4-methyl-6-{[(3R,4R)-4-{[5-(4-methylpyridin-2-yl)pentyl]oxy}pyrrolidin-3-yl]methyl}pyridin-2-amine | C22 H32 N4 O | 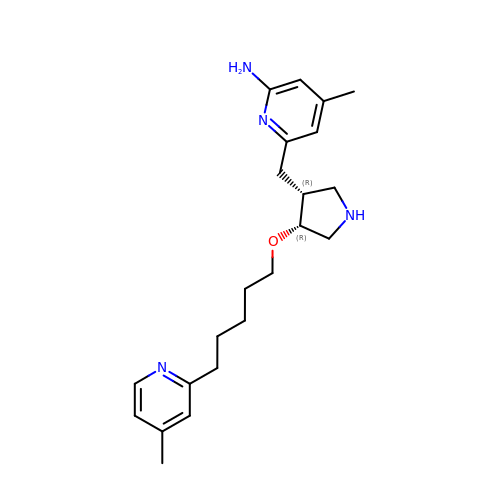ZWYPXJQSZOXLSP-NQIIRXRSSA-N In some CRISPR systems, a reverse transcriptase (RT) fusion to the Cas1 integrase and Cas6 maturase creates a single protein that enables concerted sequence integration and crRNA production. In this work, we determine the 3.7 Å resolution structure of a naturally occurring Thiomicrospira Cas6-RT-Cas1—Cas2 complex using single particle cryo-electron microscopy (cryo-EM) and investigate its activities in vitro to elucidate how RT activity might coordinate with the CRISPR integrase and with the Cas6 maturation nuclease in the context of a Cas6-RT-Cas1 fusion protein. As observed for previous CRISPR integrase structures, the Cas6-RT-Cas1—Cas2 complex is heterohexameric, consisting of a central Cas2 dimer and two distal Cas6-RT-Cas1 dimers. In this study, we identify a type III Thiomicrospira Cas6-RT-Cas1—Cas2 complex containing three active sites for CRISPR spacer integration, reverse transcription, and RNA processing, and we observe all three activities in our reconstituted system.

Approximately half of the complex displayed relatively lower local resolution, and refinement using a mask that excluded this region generated a reconstruction at 3.4 Å resolution with improved interpretability of high-resolution features. A model corresponding to two Cas2 chains and portions of four Cas6-RT-Cas1 chains was de novo built and refined into the higher resolution masked partial complex reconstruction. The Cas1 and Cas2 domains largely resemble those of the E. coli Cas1–Cas2 complex; however, there are some notable differences. When compared to the E. coli Cas1—Cas2 complex structure, the C-terminal α-helical domains of a given Cas1 are very similar (2.3 Å RMSD), while the linker and N-terminal β-sheet domains are offset by ~5–7 Å. Each Cas2 protomer has a ferredoxin-like fold, as observed in previous Cas2 structures. Additionally, the C-terminal segment (comprising amino acids 88–96) interacts with Cas1b rather than with Cas1b’ as in the E. coli Cas1—Cas2 structure. We found a cluster of residues (R832, R834, R835, and H879) adjacent to the active site that undergoes a large conformational change between Cas1a and Cas1b. In the non-catalytic Cas1b domains, these residues appear to coordinate an unknown density, potentially corresponding to a metal ion or water molecule. In the catalytic Cas1a domains, this density is not observed and the residues of interest are pushed away from each other, seemingly to accommodate the insertion of an α-helix from the RT domain.

>[2x]SNAMKHYLICFDVQHDKTRAKLSRLLEKYGPRVQGSVFEVSFKTPDRKRQLEYKIHQIIKQSNTEENNIRFYNLNKDTIKHSHDINGNPIAQLPAAIVL;>SNAMILPSFPDLTGLVVNLKFTARAEFSLNHEMAVDAFLRHSLNLGESYSHHLSIITPENGRLFYREGDTYRFVVIAMGNQQQTNSIWHTLINHLRKLPDSAPITDKQAPLRNNIKLESLNDLFDGIPVSSKESLDAYTLQRAMEQGLAWHKAANLTEQPLDIQWYWQSTVRILHADHKQHKGEQRYCRDAVQLTPLLLLKRIYETLNNVATYFGLKTNKNTTENHQAWLKEQAQYIEIQHPDLYWIDTPYFGKDAEKNTLGGMAGNFTLSLKPGIEPGLLAMLILTQMVGVGQRRTSGLGKYWLKHSLKHAHLILGLKPNRVTRSQTLLDCIIQPHIISQAIAEIEKKTNIDTLNERTLSQVQSAIGQLRKHQYQAPKLQGFTIPKKDGTERLLAVSPLYDRILQKAAAIVLTPGLDAIMSQASYGYRKGLSRQQVRYEIQNAYRQGYHWVYESDIEDFFDAVYRPQLINRLKSLLGNDPLWEQIESWLGQDIHIKDTIIERTPNLGLPQGSPLSPLLANFILDDFDSDLETHGFKIIRFADDFIILCKSQHEAQQAAHAVEQSLKEVKLSINVEKTHIIQLNQGFRFLGYLFREDHAIEIAGEKSDGRTTFAAEQTPTNLPPWLANLGTKSPQPLADDDLPKKSYGQIETQGTHLVLAGDAQIITTDNQNLIVKKDDKITHKISLEQLHAVTLIGLHTMTLPAKHRLLEHKIPVHIADRTGRYLGAVTSFQPAQNNYKNWFIQLQMCDREPFAHAIAQQIVISRIHNQRQTLLKRKAHRKQLQQTLSNLKKLQYKVTAATKRSSLNGLEGSATREYFQQFNLFLPEWAHFSKRTRRPPKDPFNVLLSLGYTILYSHTDAILQSAGFITWKGIYHQQSAAHAALASDIMESYRHLVERYAIYIINHGQIKQDDFRQEKDHLGQDTIRLSAEARRRYVGGLINRFQKFSKDKTLHQHLYQQAQQLKNAMHNQQSSQFQVWKELK[3x]>STILVIHGPNLNLLGKREPEVYGHLTLDNINRQLIAQAEQASITLDTFQSNWEGAIVDRIHQAQTEGVKLIIINPAALTHTSVALRDALLGVAIPFIEVHLSNVHAREAFRHHSYLSDKAIGVICGLGAKGYSFALDYAI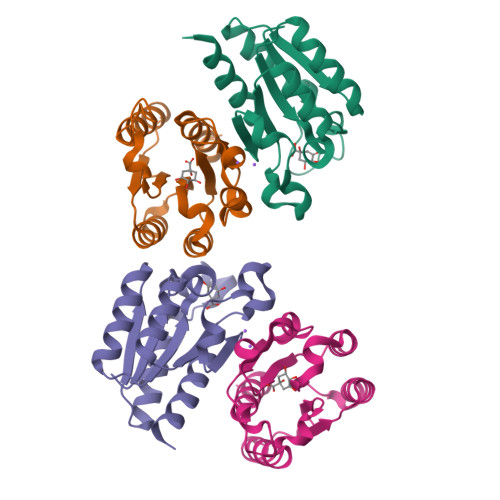EKIQPSNP[4x]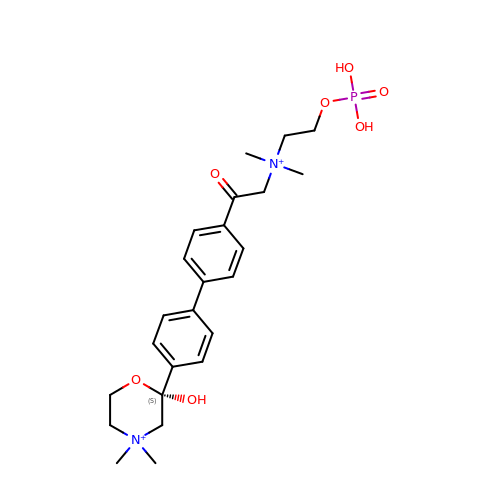(2S)-2-[4'-({dimethyl[2-(phosphonooxy)ethyl]ammonio}acetyl)biphenyl-4-yl]-2-hydroxy-4,4-dimethylmorpholin-4-ium | C24 H35 N2 O7 P | MERLSFHNUMSODQ-XMMPIXPASA-P>HGAWDEWSPWSLCSSTCGRGFRDRTRTCRPPQFGGNPCEGP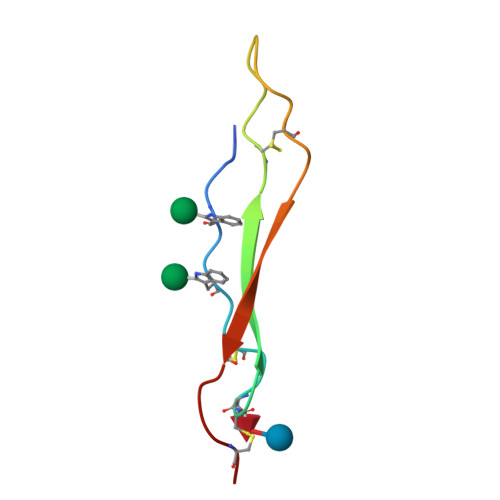EKQTKFCNIALCP[4x]> GPGSNATQINEELYRLLEDTEILNQEITEGLLKGFEVPDAGVAIQLSKRDVVYPARILIIVLSEMWRFGLTKQSESFLAQVLTTIQKVVTQLKGNDLIPSGVFWLANVRELYSFVVFALNSILTEETF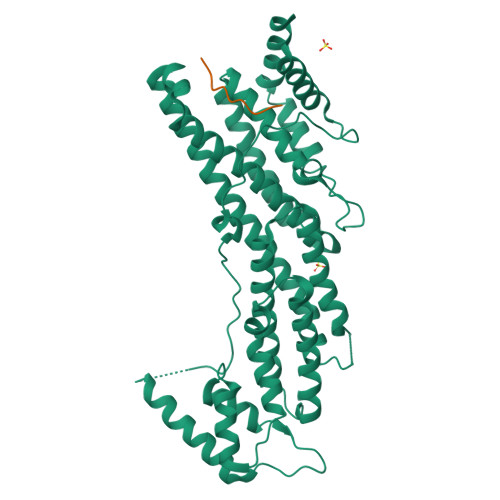KNGMTDEEYKEYVSLVTELKDDFEALSYNIYNIWLKKLQKQLQKKAINAVVISESLPGFSAGETSGANTEEYTMDDILTFFNSIYWCMKSFHIENEVFHAVVTTLLNYVDAICFNELIMKRNFLSWKRGLQLNYNVTRLEEWCKTHGLTDGTECLQHLIQTAKLLQVRKYTIEDIDILRGICYSLTPAQLQKLISQYQVADYESPIPQEILRYVADIVKKEAALSSSGNDSKGHEHSSSIFITPETGPFTDPFSLIKTRKFDQVEAYIPAWLSLPSTKRIVDLVAQQVVQDGHGSENLYFQ;> SGSGSGSGSGSEFNHGFHLDILKGRK> SMKRGRGGRVDPFEFVTYSGEEIKESSSEERVKEGANKSSPTRTRILSAALSPAERAIFDVPIEKWLSIDRSSLSGWKCAVPRPVTIEQLRPVDPSDAILRHIALYRGPVTDLQLDAIVNAANTRCLGGGGVDGAIHRVAGPLLLRECATFNGCQTGECRLTKGYQLPARYVLHTVGPVGERPDMLRKCYRSILSLALKNGLRSIGFCCVSTGVYGYPLLPATRIALGETRKFLEEHGGALDMCCFACFQEDEYKTYEKCVGKSSL

We named these proteins as Trypanosoma brucei MacroD-like protein (TbMDO) and Trypanosoma cruzi MacroD-like protein (TcMDO). We show that the trypanosomatid MacroD1/MacroD2 homologues are hydrolyzing both protein-linked ADP-ribose and free O-acetyl-ADP-ribose. The macrodomain fold (starting from residues 99 and 92 in TbMDO and TcMDO, respectively) is well-conserved between the human MacroD proteins and consists of a central mostly parallel six-stranded β-sheet surrounded by five α-helices. Active site of the macrodomains is located at the C-terminal edge of the β-sheet and is lined by N-terminal ends of four α-helices.

Crystal structures of TbMDO were determined to 1.95 Å and 1.2 Å resolution (for crystal form 1 and 2, respectively) and crystal structure of TcMDO to 2.0 Å resolution. The two crystal forms of TbMDO are almost identical with RMSD of 0.4 Å. Structures of TbMDO and TcMDO comprise residues from 11–261 and 13–257, respectively and share a highly conserved structure (RMSD 0.84 Å). While the N-terminus of the TbMDO folds back to the core and extends the β-sheet, the N-terminus of the TcMDO packs to the precisely same site but in the neighboring molecule in the crystal. When comparing the ADP-ribose bound structure to apo-TbMDO, it is evident that the binding site for ADP-ribose in TbMDO is preformed. Upon binding of ADP-ribose, eight water molecules (and a glycerol molecule) are displaced but no large conformational changes in coordinating residues are observed.>[2x]GSHMKVPTQPIPLMMNIFRDVLPTVHRYYDQWKERAKSIPDPELRAQALDALERKEFHCEGGGIYGLLARDRFDELIQFIIAYQIMCDYLDNLCDQSDYLDPKDFRSLHNALLAALTPGEPLVNYYQYRIEQEDGGYLHELIETCQHILVTFPSFRMVQENMLELSQLYGDLQVHKHVVKEERIPRLEAWFNEHKEKMPEMTWFEFSACTGSTLGVYTLATYATKEGL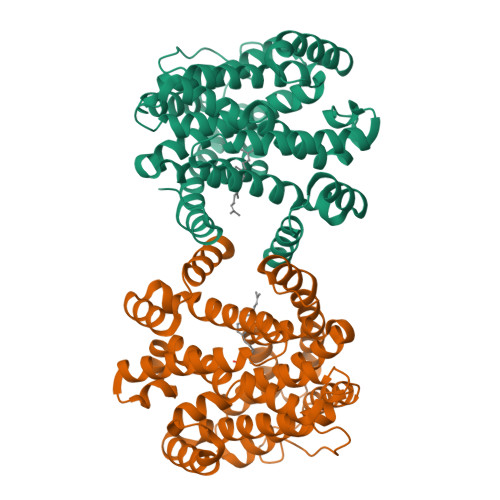TSEQADVIKAGYFPWVQGVHLLLDYFIDQEEDIADDELNFLFYYENEEQMIERFQYFVQKAEESLSTLPDPKFHRHIWRGIIAIYLSDEKVQKNKELKKKSKQMIKMGGLPSLLFYLNSWIYRRDK>MHHHHHHENLYFQGSGDESHYPEFSWDTVPIAFHFGKSQGLLTKEEAEFVATRSNFICLEKGHATRTHGTTEAGIEAEARQLKNLNPKMKVIFYWNTFLDYSMFAAHKEYAKHPQWWLRTTTGELDRKKGQLMRYDLSNAEFRNWWTNVAAKAVVDGTCDGVFMDAFPQIASQANR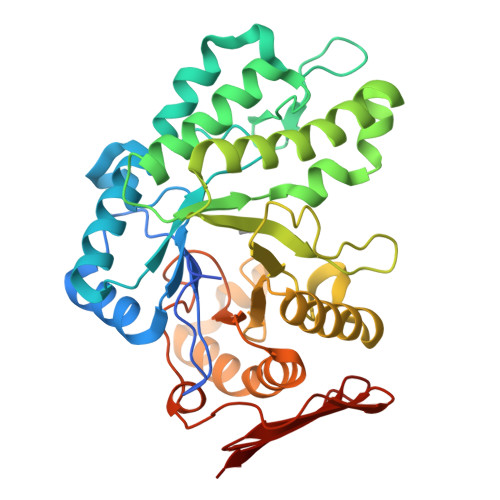KLWGDEKFEAIQQGLQDIIQETRQKIGDDKLIVYNGIRSTPDWSAGFDFAEYTDAAMIEHFGHFQSASKETMLRDILEMQRAAKAGKIVVLKGWAGFTFIDDQAMRKPLTQKRRVAKDSLKFPLACFLAGAQENCYFIYNWGYRMENGCLEWYPEFDKPLGKPVGEMVRDGWKLSREYKHASVRVDLESKEAEIRWR[6x]> LGTNYLLSGQTLDREGHLKNGDFDLVMQDDCNLVLYNGNWQSNTANKGRDCKLTLTDYGELVIKNGDGSTVWRSRAQSVKGNYAAVVHPDGRLVVFGPSVFKIDPWVPG;> NIPFTNNLLFSGQVLYGDGRLT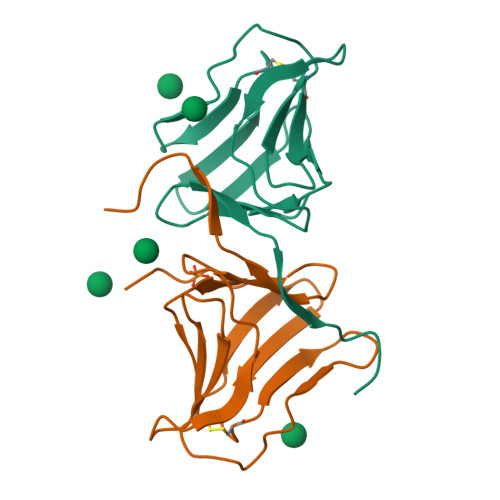AKSHQLVMQGDCNLVLYGGKYGWQSNTHGNGEHCFLRLNHKGELIIKDDDFKTIWSSSSSSKHGDYVLILRDDGFAVIYGPAIWETSPQA>MANIFLILFLFCFINFGNATPTTHNQDKTDKEEQYCVPNIEQDPQILLEQSLDAKDWALSNGLVKFVDVPTCPECGKKTKKMMTQFLPLSLYPSPFPRKLFQQAVDVQKAMLLLYFRASCDYEFLKEAHREVLNSELDNGIKKLVKRLDGMLSDGIRQPVAMFCQRADYMASQEDDGQYVLKQVEVNTGAIGSFGTTPRFSRLHRRMVSNAGIDASESVMPSDQTDTMAAETLYQAWLEFGNAEAVILFLHGSPNSHLMLESRQITHQLESISTERIKCRFITITEGLNRLKRDPNNFSLILDDKFVVAVVFDRLGGAVTKEEMDLNFVIDHSTAIKTPPYIFALSHTKRMQQVFTKPGMVEKFFNNPEEEHM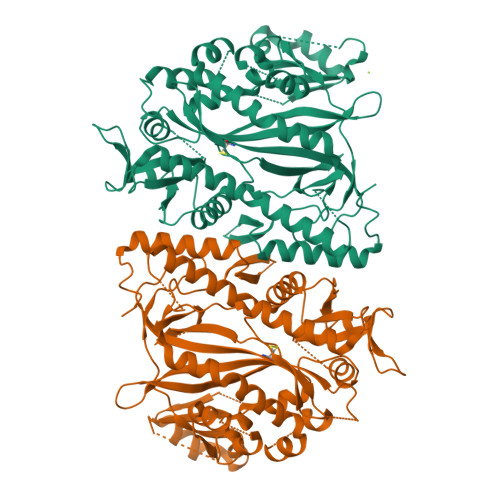AEAIRKVQTKGWAIGKDEDLTEDIIKKATENPHRYVLKNNGCSSNAADMFFNEDILKKLKTMAPADRDFYYLTEKLRPMVIKNHFVRPNMAPTLNLDATPELGIFGCLLGNMETGKVSYFSRTGHMMKSKLANVDEGGVWKGFSVYDSPYLV[2x]>[2x]GPTITETSKPTLRRIPRSAGDEAIFQVLQEDGVVVIEGFMSADQVRRFNGEIDPHMKQWELGQKSYQESYLAGMRQLSSLPLFSKL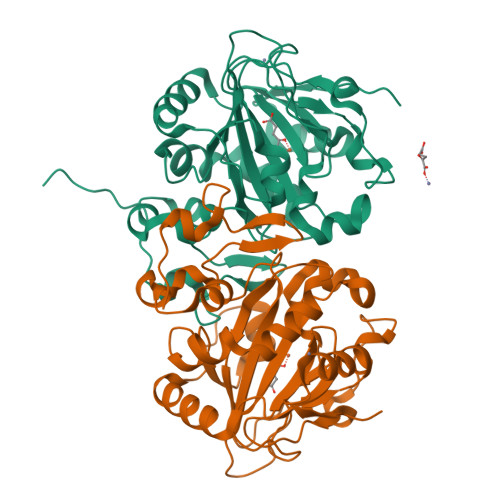FRDELMNDELLHGLCKRLFGPESGDYWLTTSSVLETEPGYHGQELHREHDGIPICTTLGRQSPESMLNFLTALTDFTAENGATRVLPGSHLWEDFSAPPPKADTAIPAVMNPGDAVLFTGKTLHGAGKNNTTDFLRRGFPLIMQSCQFTPVEASVALPRELVETMTPLAQKMVGWRTVSAKGVDIWTYDLKDLATGIDLKSNQVAKKA> KIINIGVLAHVDAGKTTLTESLLYNSGAITELGSVDKGTTRTDNTLLERQRGITIQTGITSFQWENTKVNIIDTPGHMDFLAE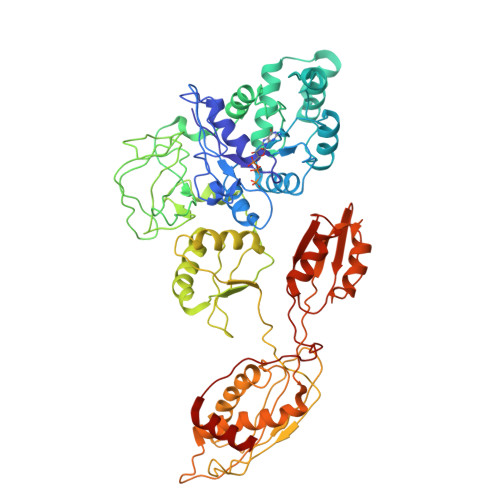VYRSLSVLDGAILLISAKDGVQAQTRILFHALRKMGIPTIFFINKIDQNGIDLSTVYQDIKEKLSAEIVIKQKVELYPNVCVTNFTESEQWDTVIEGNDDLLEKYMSGKSLEALELEQEESIRFQNCSLFPLYHGSAKSNIGIDNLIEVITNKFYSSTHRGPSELCGNVFKIEYTKKRQRLAYIRLYSGVLHLRDSVRVSEKEKIKVTEMYTSINGELCKIDRAYSGEIVILQNEFLKLNSVLGDTKLLPQRKKIENPHPLLQTTVEPSKPEQREMLLDALLEISDSDPLLRYYVDSTTHEIILSFLGKVQMEVISALLQEKYHVEIELKEPTVIYMERPLKNAEYTIHIEVPPNPFWASIGLSVSPLPLGSGMQYESSVSLGYLNQSFQNAVMEGIRYGCEQGLYGWNVTDCKICFKYGLYYSPVSTPADFRMLAPIVLEQVLKKAGTELLEPYLSFKIYAPQEYLSRAYNDAPKYCANIVDTQLKNNEVILSGEIPARCIQEYRSDLTFFTNGRSVCLTELKGYHVTTGEPVCQPRRPNSRIDKVRYMFNKIT>AGAGAMSIPSSQYGFVFNKQSGLKLRNDLPVHKPKAGQLLLKVDAVGLCHSDLHVIYEGLDCGDNYVMGHEIAGTVAAVGDDVINYKVGDRVACVGPNGCGGCKYCRGAIDNVCKNAFGDWFGLGYDGGYQQYLLVTRPRNLSRIPDNVSADVAAASTDAVLTPYHAIKMAQVSPTSNILLIGAGGLGGNAIQVAKAFGAKVTVLDKKKEARDQAKKLGADAVYETLPESISPGSFSACFDFVSVQATFDVCQKYVEPKGVIMPVGLGAPNLS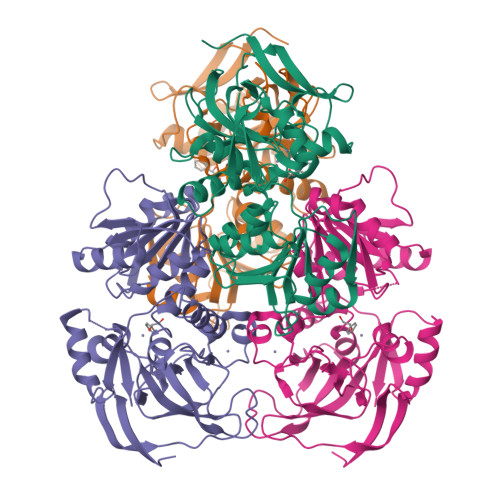FNLGDLALREIRILGSFWGTTNDLDDVLKLVSEGKVKPVVRSAKLKELPEYIEKLRNNAYEGRVVFNP[4x]5-{(3aS,4S,6aR)-1-[(benzyloxy)carbonyl]-2-oxohexahydro-1H-thieno[3,4-d]imidazol-4-yl}pentanoic 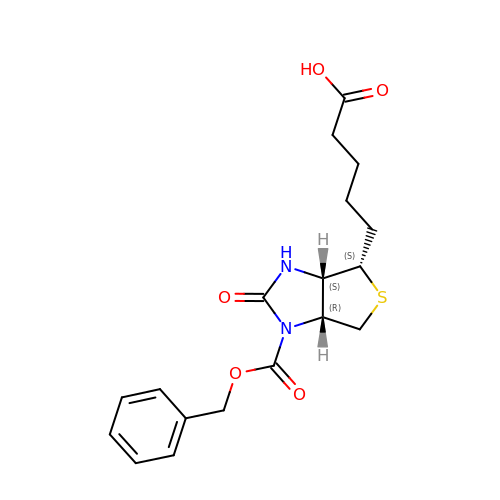acid | C18 H22 N2 O5 S | BWNGWJMPVBQLHD-DZKIICNBSA-N> ESKQIQALRYYSAQGYSVINKYLRGDDYPETQAKETLLSRDYLSTNEPSDEEFKNAMSVYINDIAEGLS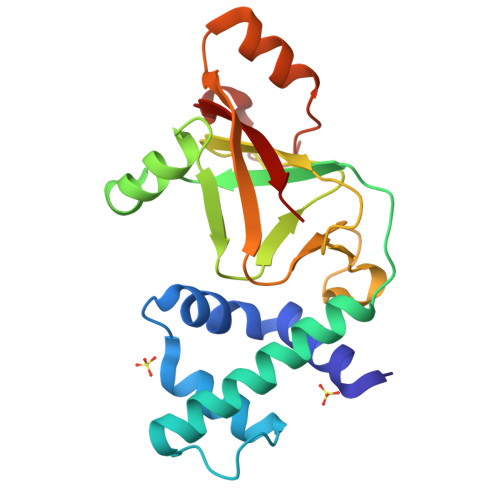SLPETDHRVVYRGLKLDKPALSDVLKEYTTIGNIIIDKAFMSTSPDKAWINDTILNIYLEKGHKGRILGDVAHFKGEAEMLFPPNTKLKIESIVNCGSQDFASQLSKLRLSDDATADTNRIKRIINMRVLN> MGHHHHHHSHMADNMTTTQIEVGPGATNATINFEAGILECYERFSWQRALDYPGQDRLHRLKRKLESR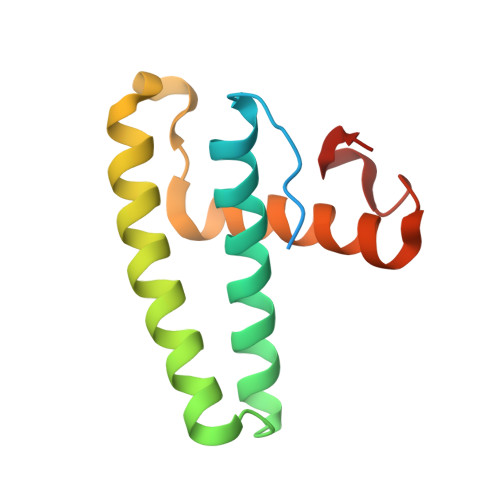IKTHNKSEPENKRMSLEERKAIGVKMMKVLLFMDPSAGIEGFEPY> MRNKIFISHATPEDDDFTRWLSLKLIGLGYEVWCDILFLDKGVDFWSTIEKEIRENTCKFLIVSSTAGNKREGVLKELAVATKVKKHLQDDMFIIPLAIDENLSYDDINIEIVRLNAIDFKKSWAKGLQDLLDAFEKQNVPKKPPDHSKSNLLYQQIFLHDKQAIEKEETYDSNWFPIISFPNELRFHRYDWRLPKQFDVRTLAFPAIRYKEYLCTFAWEYDFIHQLPKTETYNGQESIRISTSDILSGRYDTDFIRNYECQRLIVQLINKAFELRMKDKNVREYQMSKTFAYWIEKGKLEKDKFEKIKLVGKQKNKYWHFGISAAGKLYPSPVLMVSSHIIFTMDGINLIKSKSIQHS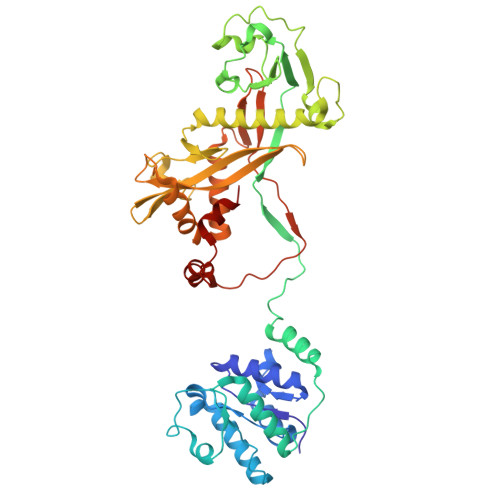SRRKQGKNWWNDKWREKLLAFIRFLSDDQNAIYLNVGSEEKILISNKPLKFFGKMSYVTPSEVTLEEESVLADINNFEEDTEDLDELEDIE>[2x]GPLGSIKELKMSKDEIKREYKEMEGSPEIKSKRRQFHQEIQSRNMRENVKRSSVVVAN;>PTHIAIGILYKRGETPLPLVTFKYTDAQVQTVRKIAEEEGVPILQRIPLARALYWDA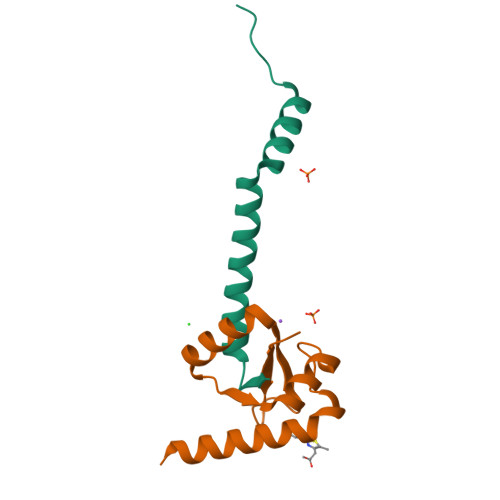LVDHYIPAEQIEATAEVLRWLERQNIEKQHSEML[2x]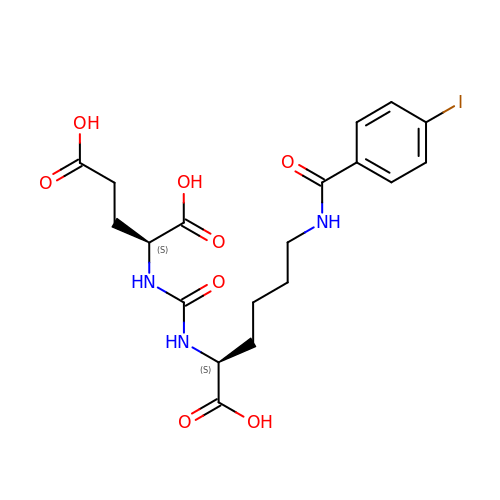N-{[(1S)-1-carboxy-5-{[(4-iodophenyl)carbonyl]amino}pentyl]carbamoyl}-L-glutamic acid | C19 H24 I N3 O8 | ROXRILBFJQYPNZ-KBPBESRZSA-N>[4x]MAVYHMTPPSGWLCDPQRPVTTHGAYQLYYLHSDQNNGPGGWDHASTTDGVAFTHHGTVMPLRPDFPVWSGSAVVDTANTAGFGAGAVVALATQPTDGVRKYQEQYLYWSTDGGFTFTALPDPVIVNTDGRAATTPAEIENAEWFRDPKIHWDTARGEWVCVIGRLRYAAFYTSPNLRDWTLRRNFDYPNHALGGIECPDLFEITADDGTRHWVL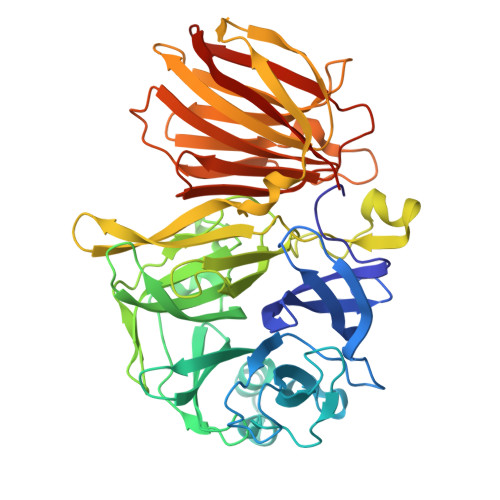AASMDAYGIGLPMTYAYWTGTWDGEQFHADDLTPQWLDWGWDWYAAVTWPSIDAPETKRLAIAWMNNWKYAARDVPTDASDGYNGQNSIVRELRLARQPGGWYTLLSTPVAALTNYVTATTTLPDRTVDGSAVLPWNGRAYEIELDIAWDTATNVGISVGRSPDGTRHTNIGKYGADLYVDRGPSDLAGYSLAPYSRAAAPIDPGARSVHLRILVDTQSVEVFVNAGHTVLSQQVHFAEGDTGISLYTDGGPAHFTGIVVREIGQAIGSHHHHHH>[3x]GPMVLQAQEIMTQNVVTIRGSATVADAVKLMKEKKLRGLIVEPRHEQDPYGIVTETDIVYKVAAFGHDPKTMRVYEIMAKPCVVVNPELGVEYVARLFAQTRIRR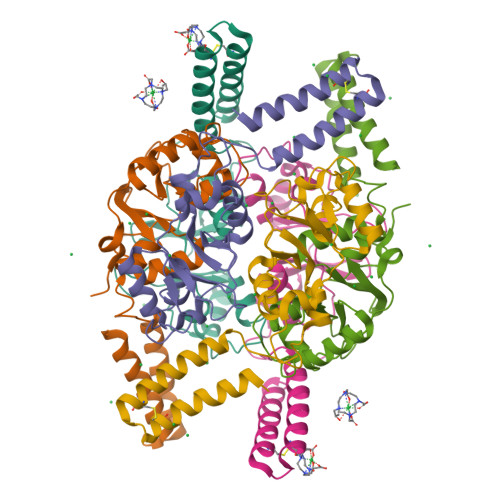APVIQGKTLLGIISVSDILFKSDFVEKPKRLFIEDEIEAAREDARAICAAKGETSPDCAAAWDVVEELQAEASHQRAKKQGSNSFQAYCEANPDALECRIYDD> GPLGSQAEVNIGMVGHVDHGKTSLTKALTGVWTDRHSE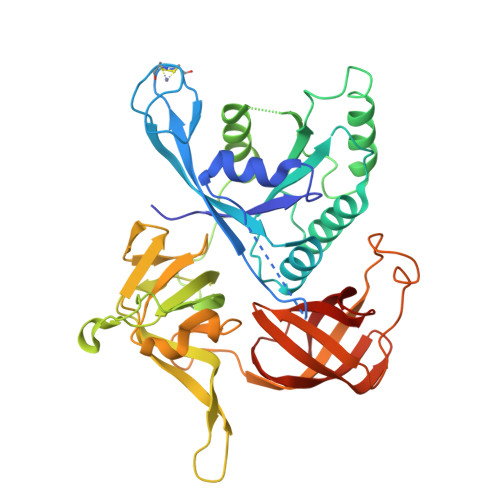ELRRGISIRLGYADCEIRKCPQCGTYTTKPRCPNCLAETEFLRRVSFVDSPGHETLMATMLSGASLMDGAILVIAANEPCPQPQTKEHLMALEILGIDKIIIVQNKIDLVDEKQAEENYEQIKEFVKGTIAENAPIIPISAHHEANIDVLLKAIQDFIPTPKRDPDATPRMYVARSFDINKPGTEIKDLKGGVLGGAIIQGVFKVGDEIEIRPGIKVTEGNKTFWKPLTTKIVSLAAGNTILRKAHPGGLIGVGTTLDPYLTKSDALTGSVVGLPGTLPPIREKITIRANLLDRVVGTKEELKIEPLRTGEVLMLNIGTATTAGVITSARGDIADIKLKLPICAEIGDRVAISRRVGSRWRLIGYGTIEG D-glucal 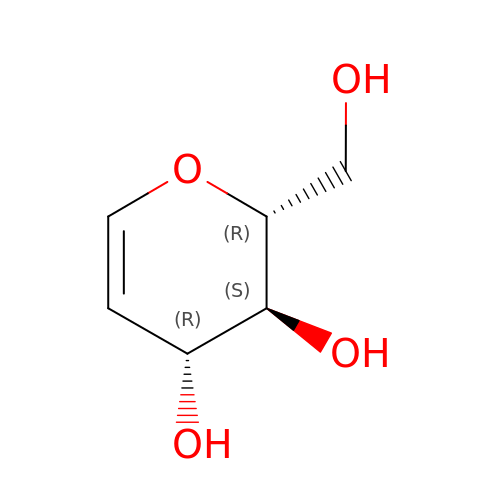| C6 H10 O4 | YVECGMZCTULTIS-PBXRRBTRSA-N>GPLGSEEGLFSQKSFLVLGFSNENESNIANIIKENAGKIMSLLSRTVADYAVVPLLGCEVEAT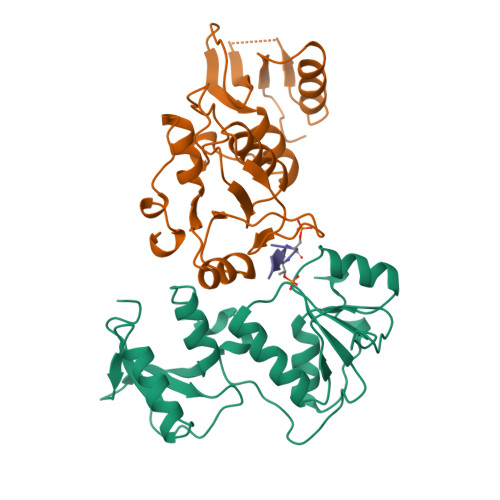VGEVVTNTWLVTCIDYQTLFDPKSNPLFTPVPVMTGMTPLEDCVISFSQCAGAEKESLTFLANLLGASVQEYFVRKSNAKKGMFASTHLILKERGGSKYEAAKKWNLPAVTIAWLLETARTGKRADESHFLIENSTKEER[4x];>[2x]GFIDSDTDVEEE> MGHHHHHHMKLTPELTPFVLFTGFEPVQVQQYIKKLYILGGEVAESAQKCTHLIASKVTRTVKFLTAISVVKHIVTPEWLEECFRCQKFIDEQNYILRDAEAEVLFSFSLEESLKRAHVSPLFKAKYFYITPGICPSLSTMKAIVECAGGKVLSKQPSFRKLMEHKQNSSLSEIILISCENDLHLCREY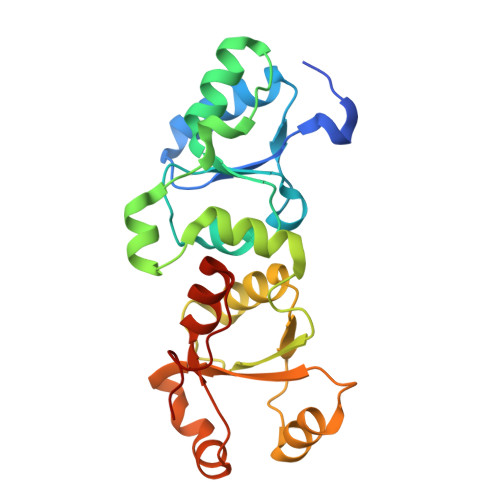FARGIDVHNAEFVLTGVLTQTLDYESYKFN> GSH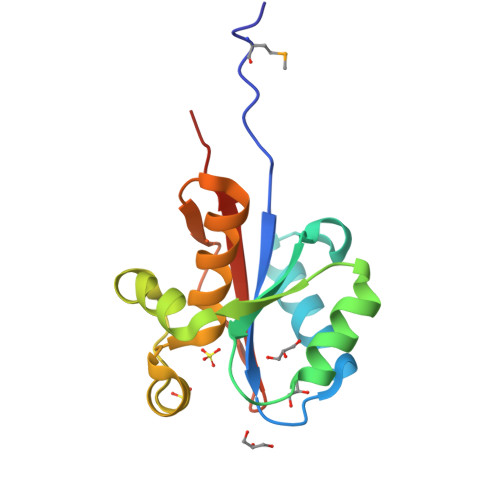MPLPIPSLLIAGIGCRRGCSAEHLRALLERTLGEHGRSLAELDALASIDGKRDEPGLRQLATLLERPVHFLAPAVLHDYEPRLLSPSAVALRETGCSSVAEAAALALAERLGGGRADLLGAKRSDDRASIALARLLTERELP butanoic acid | C4 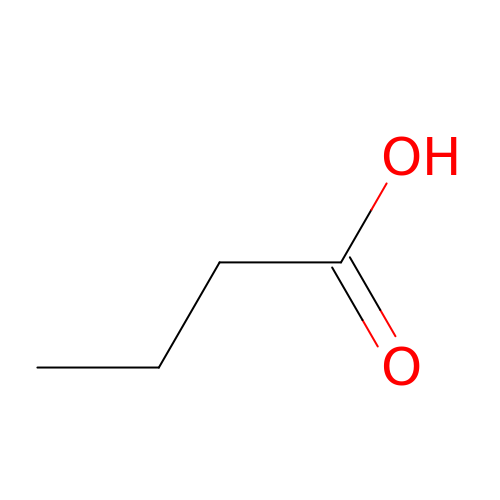H8 O2 | FERIUCNNQQJTOY-UHFFFAOYSA-N>[3x]XRMKQIE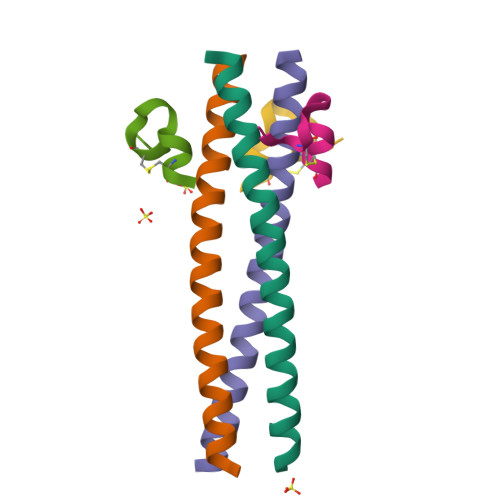DKIEEIESKQKKIENEIARIKKLLQLTVWGIKQLQARILX;>[3x]XKGACDYPEWQWLCAAX3-[4-[(4-~{tert}-butylphenyl)carbonylamino]phenyl]propanoic acid | C20 H23 N O3 | 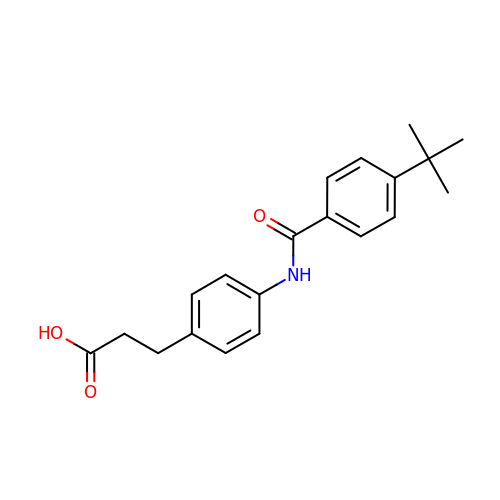IMRDLYFNSFXCTK-UHFFFAOYSA-N> ELTPDQQTLLHFIMDSYNKQRMPQEITNKILKEEFSAEENFLILTEMATNHVQVLVEFTKKLPGFQTLDHEDQIALLKGSAVEAMFLRSAEIFNKKLPSG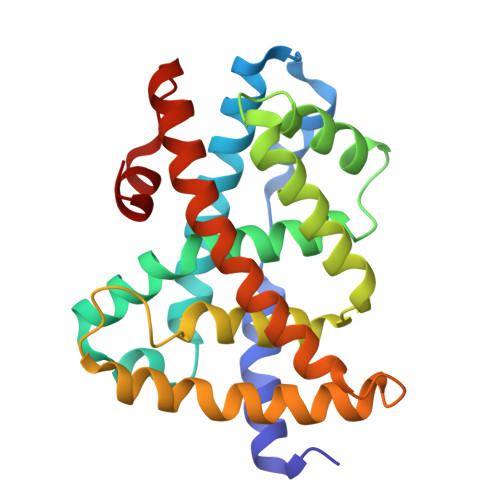HSDLLEERIRNSGISDEYITPMFSFYKSIGELKMTQEEYALLTAIVILSPDRQYIKDREAVEKLQEPLLDVLQKLCKIHQPENPQHFAELLGRLTELRTFNHHHAEMLMSWRVNDHKFTPLLEEIWDV Previously, we identified Pseudoalteromonas arctica PAMC 21717 from the Polar and Alpine Microbial Collection (PAMC) as a microbe of interest because it secretes a high level of a psychrophilic alkaline serine protease. Preliminarily, the domain structure of the translated pro21717 gene was predicted based on the results of the sequence alignments and secondary structure predictions. This analysis showed that the Pro21717 protease precursor consists of four functional domains: a signal peptide (residues 1–27), an N-terminal prosequence (residues 28–142), a catalytic domain (residues 145–483), and two β-sandwich domains (residues 489–593 and 611–708). CD-Search was used to identify the catalytic domain to either the Peptidase S8 family or the serine endo- and exo-peptidase clans of subtilases containing three conserved amino acid residues (Asp185, His244, and Ser425) that constitute a catalytic triad like that found in trypsin-like proteases.

Here, we describe the crystal structure of the catalytic domain of Pro21717 at 1.4 Å resolution. During refolding of the precursor protein, an active protease (Pro21717-CD, residues 145–483) was produced by intramolecular cleavage of the precursor. In the asymmetric unit, one Pro21717-CD molecule was found, which had a classical subtilisin-like fold consisting of 10 α-helices and 8 β-strands. Pro21717 contains three disulfide bonds (Cys207–Cys254, Cys296–Cys333, and Cys439–Cys442) and four calcium-binding sites that may influence protein stability. The fourth calcium-binding site is unique to Pro21717 and does not appear in other subtilisin-like proteases that have been structurally characterized to date. The CaIV ion in Pro21717-CD is stabilized by Asp385, Glu451, the carbonyl O atom of Val362, and two water molecules. The predicted active site containing the catalytic triad residues (Asp185, His244, and Ser425) is located at the C-terminal end of the β-sheet and forms a deep elongated pocket. The conformation of this density could clearly be identified as a small peptide bound to the predicted substrate-binding site (S2–S3–S4). Thus, the final model structure of Pro21717-CD contains only three alanine peptides in the substrate-binding site. One of the distinctive features of Pro21717-CD compared with the AprB2 protease is a loop deletion (α4–α5 loop) and a loop insertion (β6–β7 loop; residues 391–401) near the active site cleft that produces a cap structure covering the deep hydrophobic substrate-binding pocket in Pro21717-CD.

> STPNDPRFDDQWHYYEQAGGLNLPTAWDTATGSGVVVAVLDTGYRPHADLNANILPGYDMISNLSVANDGGGRDSDARDPGDAVAANECGTNGAQNSSWHGTHVAGTVAAVTNNGEGVAGVAYNAKVVPVRVLGKCGGLTSDIADGIIWASGGSVSGIPANSNPADVINMSLGGSGSCSSTTQNAINTARSNGTVVVIAAGNDNDNSANYNPGNCNGVVNVASVGRNGGRAYYSNYGSNIDVAAPGGAQSFANDSEGVLSTYNSGSSTPSSDSYGYSQGTSMAAPHVAGVAALIKQAKPDATPDEIESILKSTTRSFPATCTSCGTGIVDAAAAVAAASKGHHHHHH> SSNAIDFPFAHEDVVQKTVDDVRTLSNMSAAADQGVHDVNHSSKTLAERYKDDITALAVLPPRVDEFAKSFNDILWAGRTSATHGVSRITDFVDVTVVGIVEDIKTPEDRDEAVIELNAIAGQKSKPVDGFPGATRRLDGIWNTSSTDAANIAKVLAEATDIEKTVKELTTAFSPAKAGYKKVQEALRAYASSITKLAAAL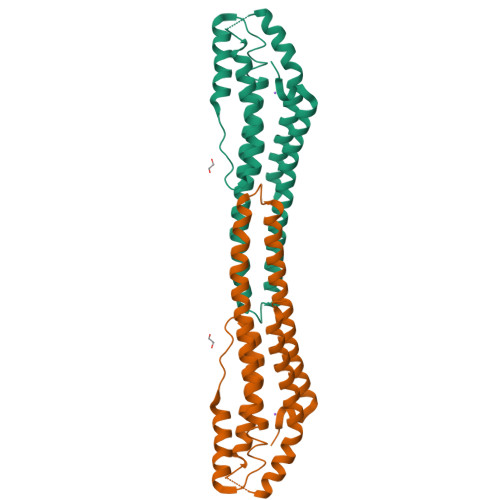EHHHHHH> MKKHHHHHHGSERTGTQPLGVQGLTEEQRMMIRELMDAQMKTFDTTFSHFKNFRLPGVLSSGCELPESLQAPSREEAAKWSQV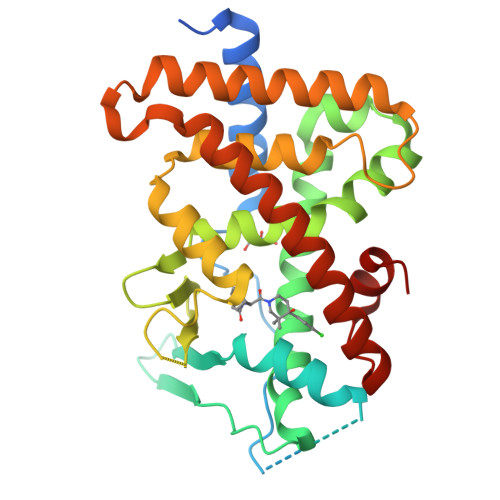RKDLCSLKVSLQLRGEDGSVWNYKPPADSGGKEIFSLLPHMADMSTYMFKGIISFAKVISYFRDLPIEDQISLLKGAAFELCQLRFNTVFNAETGTWECGRLSYCLEDTAGGFQQLLLEPMLKFHYMLKKLQLHEEEYVLMQAISLFSPDRPGVLQHRVVDQLQEQFAITLKSYIECNRPQPAHRFLFLKIMAMLTELRSINAQHTQRLLRIQDIHPFATPLMQELFGITGS> G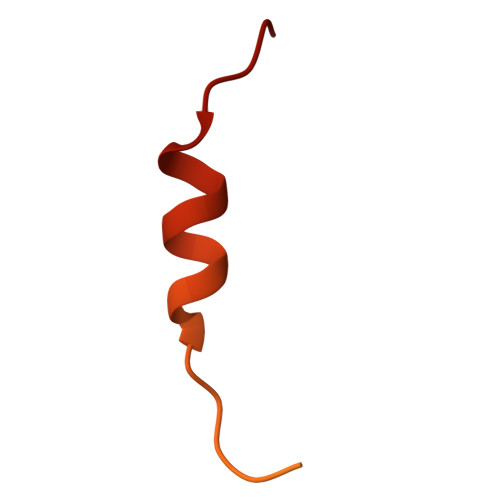SGGGPGGSHMGGNYGDDRRGGRGGYDRGGYRGRGGDRGGFRGGRGGGDRGGFGPGKMDSRGEHRQDRRERPY> GAGA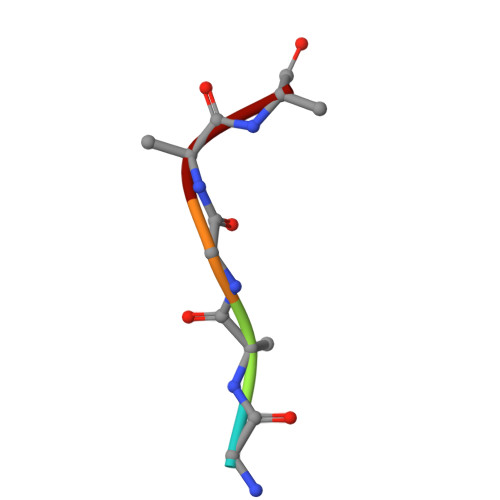A[[(2~{R},3~{S},4~{R},5~{R})-5-(6-aminopurin-9-yl)-3,4-bis(oxidanyl)oxolan-2-yl]methoxy-oxidanyl-phosphoryl] 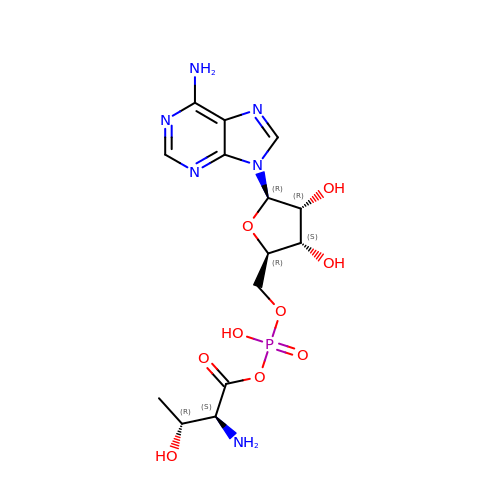(2~{S},3~{R})-2-azanyl-3-oxidanyl-butanoate | C14 H21 N6 O9 P | YYBNSQASHCKPHX-DWVDDHQFSA-N> GDRVADVIESSIGDSVSRALTQALPAPTGQNTQVSSHRLDTGEVPALQAAEIGASSNTSDESMIETRCVLNSHSTAETTLDSFFSRAGLVGEIDLPLEGTTNPNGYANWDIDITGYAQMRRKVELFTYMRFDAEFTFVACTPTGQVVPQLLQYMFVPPGAPKPESRESLAWQTATNPSVFVKLTDPPAQVSVPFMSPASAYQWFYDGYPTFGEHKQEKDLEYGACPNNMMGTFSVRTVGSSKSKYPLVVRIYMRMKHVRAWIPRPMRNQNYLFKANPNYAGNSIKPTGTSRSAITTL;> SDRVAQLTIGNSTITTQEAANIIVGYGEWPSYCSDDDATAVDKPTRPDVSVNRFYTLDTKLWEKSSKGWYWKFPDVLTETGVFGQNAQFHYLYRSGFCIHVQCNASK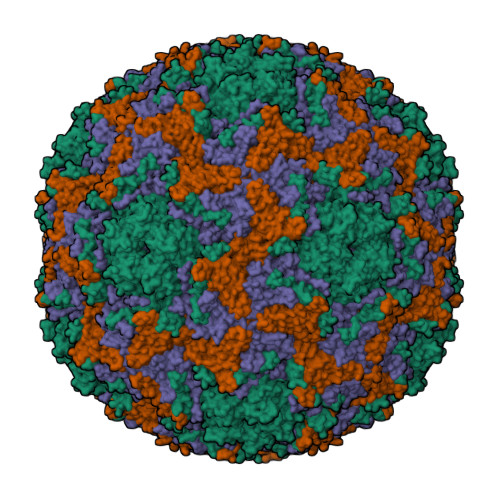FHQGALLVAILPEYVIGTVAGGTGTEDSHPPYKQTQPGADGFELQHPYVLDAGIPISQLTVCHHQRINLRTNNCATIIVPYMNTLPFDSALNHCNFGLLVVPISPLDFDQGATPVIPITITLAPMCSEFAGLRQAVTQ;> GFPTELKPGTNQFLTTDDGVSAPILPNFHPTPCIHIPGEVRNLLELCQVETILEVNNVPTNATSLMERLRFPVSAQAGKGELCAVFRADPGRDGPWQSTMLGQLCGYYTQWSGSLEVTFMFTGSFMATGKMLIAYTPPGGPLPKDRATAMLGTHVIWDFGLQSSVTLVIPWISNTHYRAHARDGVFDYYTTGLVSIWYQTNYVVPIGAPNTAYIIALAAAQKNFTMKLCKDTSHILQTASIQ;> MGSQVSTQRSGSHENSNSATEGSTINYTTINYYKDSYAATAGKQSLKQDPDKFANPVKDIFTEMAAPLKSPSAEACGY>MFYINSKYKIDLDKIMTKMKNKSVINIDDVDDEELLAILYTSKQFEKILKNNEDSKYLENKVFCSVFLEPSTRTRCSFDAAILKLGSKVLNITDMNSTSFYKGETVEDAFKILSTYVDGIIYRDPSKKNVDIAVSSSSKPIINAGNGTGEHPTQSLLDFYTIHNYFPFILDRNINKKLNIAFVGDLKNGRTVHSLSKLLSRYNVSFNFVSCKSLNIPKDIVNTITYNLKKNNFYSDDSIKYFDNLEEGLEDVHIIYMTRIQKERFTDVDEYNQYKNAFILSNKTLENTRDDTKILHPLPRVNEIKVEVDSNPKSVYFTQAENGLYVRMALLYLIFSSTSSAWSHPQFEK[3x]

Aspartate transcarbamoylase (ATC) catalyzes the second step of de novo pyrimidine synthesis, combining l-aspartate (l-ASP) and carbamoyl phosphate (CP) to form carbamoyl-aspartate (CP-ASP) and phosphate. Aspartate transcarbamoylase (ATC) has been suggested to be a promising target for antimalarial drug development. In depth structural analysis of the ATC catalytic cycle has been performed previously, which indicated that ATC exists in a low substrate affinity “T” state and a high substrate affinity “R” state. Here, we describe a series of small-molecule inhibitors of P. falciparum ATC with low nanomolar binding affinities that selectively bind to a previously unreported allosteric pocket, thereby inhibiting ATC activation.

Fragments A, B, C, and D bind in a buried hydrophobic cavity formed by the α3 helix, α4 helix, and β1–3 sheets of the adjacent subunit. Enzymatic assays indicated an IC50 for these compounds of 10, 125, 150, and 145 μM, respectively. In the citrate-PfATC complex, both Ser135 and Lys138 from 120 s loop form polar contacts with phosphate (which represents the product of PfATC) to support the 120 s loop in the closed position, whereas in the Fragment A:PfATC complex, Ser135 and Lys138 adopt an open conformation, forming a hydrophobic region buried under the 120 s loop that accommodates Fragment A. The 120 s loop of the citrate-bound PfATC showed a significant shift compared to the Fragment A-bound structure between the α-carbons of Ser135 in the two structures (7.8 Å). Further analysis revealed that the amino group of Fragment A forms polar contact with Phe136 and a water-mediated bridge with the main chain of Ser107. The main aromatic ring faces the Arg109-Glu140 pair, with which the fragment forms a cation−π interaction. Fragment A blocks the motion of the 120 s loop and holds PfATC in its T-state—preventing the movement of the Asp domain and CP domain toward each other to form the carbamoyl aspartate and phosphate. Structural alignment of Fragment A:PfATC and apo-PfATC structures did not show any significant impact on the structure of PfATC. However, stabilizing effects of Fragment A were confirmed by DSF experiments.>MPGVVEELVAAIGAEQVVTDPAVMEGYSHDEAEWAPYDAPAAVVRPRDTADVAEVVRICAGRGVAVVGRGAGTGLSGAANAGRGWVVVSFERMNRVLEVDTVQQTVTVQPGVVNDDLRARVAQDGLWYPPDPASSPWSTIGGNVATNAGGLCCVKYGVTRDYVLGMEAVVGSGEVVRLGRTTAKGVTGYDLAGLMVGSEGTLGLVTEVTLRLVPLRRGVEHTVVGYFDSLTDAGRAVAAVSAAGIVPSALELIDRFCLQAVDEWKNMGLSAEGEVLLLARSDLPGTSGQEEADRILECFEKEKAVYAVRSTDEEEAEALFQARRLAYPALERLGPLLTEDVCVPKARVPHMLEAIEAAGERFDTRIGNIAHAGDGNLHPLFIVPAGDEEAKRRAKQAFEVIVDEALAVGGTVTGEHGVGLLKMRGAADELGPHVLAMHRAVKGALDPAGIFNPGKVFALEEERD[8x]

Here, we report the discovery and characterization of a new FAD-dependent D-lactate dehydrogenase (PdG-D-LDH) from the gut microbiome of the isopod Porcellio dilatatus. PdG-D-LDH exhibits a strong catalytic preference toward D-lactate and preferentially reduces quinones over cytochrome c or molecular oxygen. X-ray crystallography revealed a VAO/PCMH-like fold with a solvent-accessible active site that harbors both a FAD cofactor and an Fe(II) ion. PdG-D-LDH exhibits the characteristic VAO/PCMH structural fold.

The crystal structure of the enzyme was solved both in the absence or presence of D-lactate (PdG-D-LDH–lactate), revealing a Cα root-mean-square deviation (RMSD) of 0.46 Å between the two structures. The structure contains a non-covalently bound FAD at the active site. The active site located at the interface of the FAD- and substrate-binding domains is connected to the solvent by a cavity with a volume of 314.6 Å3 and an area of 490.5 Å2. The substrate-binding domain binds an Fe(II) ion coordinated by strictly conserved residues: two histidines (H371, H378) and one glutamate (E415). The iron ion forms a hydrogen bond with the FAD O4 atom. The B-factor values of the substrate-binding domains are higher (36–126 Å2) than those of the other domains (25–85 Å2), indicating greater flexibility, which may play a role in binding substrates, product release, and catalysis. Unlike many other members of the VAO/PCMH family, the FAD cofactor is not covalently attached to the enzyme, as it was released upon chemical treatment with SDS.> MASEALTMIVNLLRSQRPLQEPTVEQMRAGL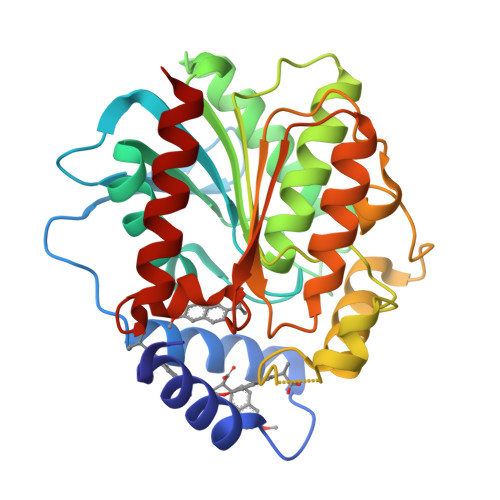EAMAQMSPLPADVELTTVDAGGVPGAWVRVPESDPDRVVLYLHGGGYVIGSIRTHRDLAQRIARAARCRVLLIDYRLAPEHPHPAAVEDSTRAYRWLLETGSDPKRMAIAGDSAGGGLTVATLVALRDAGVPLPAAAVCLSPWVDLEGIGESMTTKAAVDPMVQREPLLRMASMYLAGQDPRTPLAAPLYADLRGLPPLLIQVGTAETLLDDSVRLAERARAAGVQVTLEPWEDMIHVWQAFAAMLPEGQQAIERIGEFLRQHWQ>[8x]MKKLCFALVMLLSCVCSYAQTITTYSLSEAPITKEELLKGNLKVALRVWTTSKDLYLSNANNSNAFDANGSTVFAVEAVKGGVKLKNVKSNEYFGGEGAALARTADAAKAKVFSPVKIGSKVANTH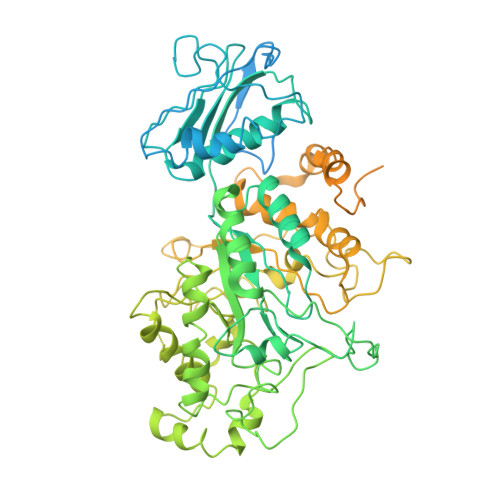ADADETRSFWITCQAGGTKYLNTNTSNNATVQYAGGNGNWSTFYIYKVSEEQIAVPYPTCIIPAPRGAELNGEGRLALSAMDNISFTTDPALAEEAYVLNITADGISVASSTEKGKFYALQSLAQLAEGNAEGLPLVRIADKPRFGYRGFMLDVSRHFFSVAEVKKMIDIMARYKMNVFHWHLTDDQGWRAEIKRYPKLTTVGATRSDNYDTPITKIEENGQVYWTGNGAKTGKPYGPYFYTQDEMREVVAYAKERHIEVLPEVDMPGHFVAAMAAYPEYSCNPSRAPQVWTGGGISSDVLNVANPQAVEFAKNILDELCDIFPYPYIHVGGDECPTTQWEHNDLCQQKYKELGLTSYRQLQAHFIKDLADFVATKNKHLVCWNEAITAGGADLDLMKQTQSTIMSWNPCQEGVAKAVKKLGLPAIVTEYHKGDGGYYICRKQSNDYGEPSGAGYGNDGVEGCYNYVPVQGMYTQEQMALVKGVQGTFWTEHVGTNEYLEYLALPRLICVAEAGWTPQVFKNWDNFRTRLANQTQWLDDHGYVYARHWMPGYVPRTQPMPENEKVAATPELSSLKSPKWYRIKFTAGGTYLQMNGSNLSTNALFQNDKSQYYAIIPTSTKKPSLSSVKLYSANGYWVTTKEGTATNGQSGTFVCGTESEAKALYLNLQKHTADTQKWVITKIADKTTGFNTWGGDNPGANIGFWNVNSNSDKVEFTTDDYNAGVDTAIGTIKADDAHNNLTAAVYNAQGMRLNGMQQGLNVVLFADGTAQKVFMK>[6x]IPDGVVSALSLRERIREHLSSEESVGLLFSGCTGINDKTLGARGGEVIMVTSGSGMGKSTFVRQQALQWGTAMGKKVGLAMLEESVEETAEDLIGLHNRVRLRQSDSLKREIIENGKFDQWFDELFGNDTFHLYDSFAEAETDRLLAKLAYMRSGLGCDVIILDHISIVVSASGESD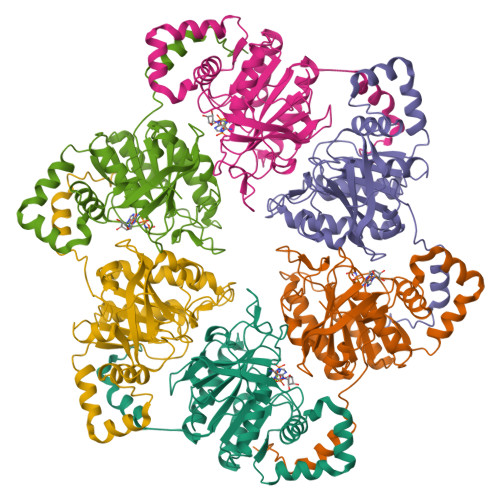ERKMIDNLMTKLKGFAKSTGVVLVVICHLKNPDKGKAHEEGRPVSITDLRGSGALRQLSDTIIALERNQQGDMPNLVLVRILKCRFTGDTGIAGYMEYNKETGWLEPSSYSG>SGKIIGIDLGTTNSCVAIMDGTTPRVLENAEGDRTTPSIIAYTQDGETLVGQPAKRQAVTNPQNTLFAIKRLIGRRFQDEEVQRDVSIMPFKIIAADNGDAWVEVKGQKMAPPQISAEVLKKMKKTAEDYLGEPVTEAVITVPAYFNDAQRQATKDAGRIAGLEVKRIINEPTAAALAYGLDKGTGNRTIAVYDLGGGAFDISIIEIDEVDGEKTFEVLATNGDTHLGGEDFDSRLINYLVEEFKKDQGIDLRNDPLAMQRLKEAAEKAKIELSSAQQTDVNLPYITADATGPKHMNIKVTRAKLESLVEDLVNRSIEPLKVALQDAGLSVSDIDDVILVGGQTRMPMVQKKVAEFFGKEPRKDVNPDEAVAIGAAVQGGVLTGDVKDVLLLDVTPLSLGIETMGGVMTTLIAKNTTIPTKHSQVFSMGGAV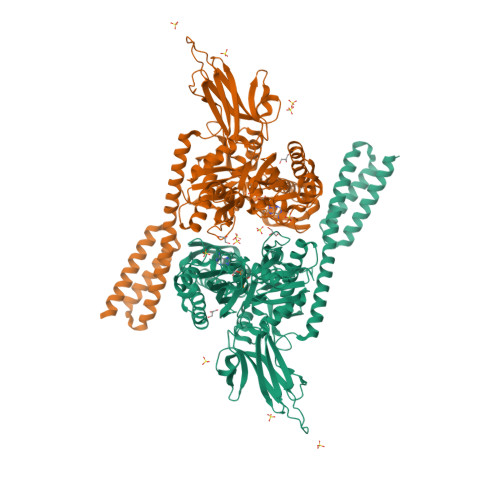TIHVLQGERKRAADNKSLGQFNLDGINPAPRGMPQIEVTFDIDADGILHVSAKDKNSGKEQKITIKASSGLNEDEIQKMVRDAEANAEADRKFEELVQTRNQGDHLLHSTRKQVEEAGDKLPADDKTAIESALTALETALKGEDKAAIEAKMQELAQVSQKLMEIAQQQHAQQQHA[2x]>[4x]GSSHHHHHHSSGLVPRGSHMSSRLEREAARRRTFAIISHPDAGKTTLTEKLLLFGGAIQMAGSVKARKAARHATSDWMAMERERGISVTTSVMQFPYRDRVVNLLDTPGHQDFSEDTYR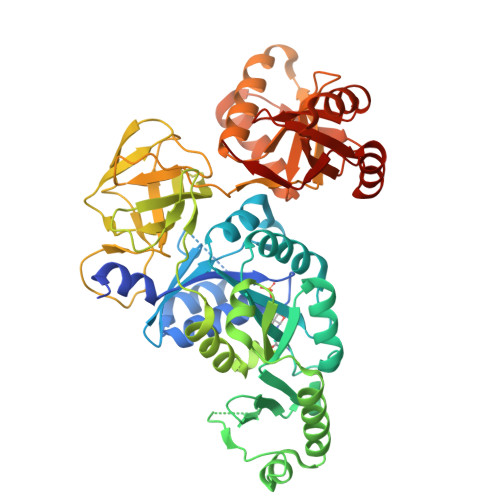VLTAVDSALVVIDAAKGVEAQTRKLMDVCRMRATPVMTFVNKMDREALHPLDVMADIEQHLQIECAPMTWPIGMGSSFKGTYDLLHKQLHLFSATHGGRIQSGIVIHGADDPQLDEYLGDQAEQLRMDLALLEEAGTPFDEERYLKGELTPVFFGSAINNFGVREMLDMFVEFAPGPQPRPAATRVVEPGEEAFTGVVFKIQANMDKAHRDRMAFLRICSGTFTRGMRLKHHRTGKDVTVANATIFMAQDRTGVEEAFPGDIIGIPNHGTIKIGDTFTESKEVLKFVGIPNFAPEHFRRVRLKNPLKAKQLQKGLEQLAEEGAVQLFRPLVNNDYILGAVGVLQFDVIVARLADEYGVDAVYEGVSTHTARWVYCEDKKIFADFQDYHRGELAVDAEGALAYLAPNPWRLESAMERYPKVEFRTTREIS>[4x]SNAMFERFDSDRSRYASLGVVSSLPSGLIDSIWLIIDLNLKGV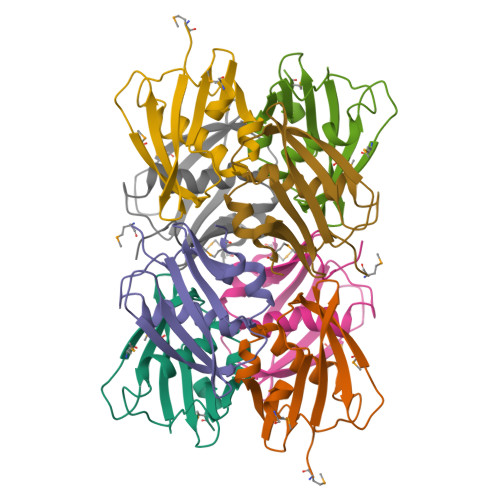IPLNDLLHFDLLNNNGKVTVHFSQENSSVEMAIDLPFSYSTAYPSRIFAFDDGHRETILLPAEMLES> MKIFFITSNPGKVREVANFLGTFGIEIVQLKHEYPEIQAEKLEDVVDFGISWLKGKVPEPFMIEDSGLFIESLKGFPGVYSSYVYRTIGLEGILKLMEGAEDRRAYFKSVIGFY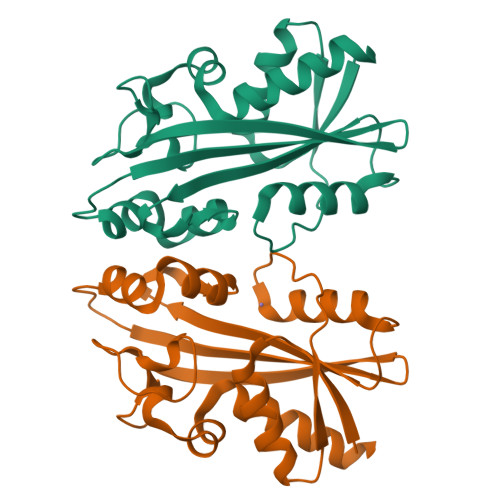IDGKAYKFSGVTWGRISNEKRGTHGFGYDPIFIPEGSEKTFAEMTIEEKNALSHRGKALKAFFEWLKVNLKY The bacterial periplasmic methionine‐binding protein MetQ is involved in the import of methionine by the cognate MetNI methionine ATP binding cassette (ABC) transporter. MetQ, the substrate‐binding protein (SBP) for MetNI,5, 6 is proposed to play a dual role in transport by either binding l‐methionine for delivery to the translocation pathway of MetNI, or by facilitating d‐methionine uptake through the ligand‐free form when complexed to the transporter. Structural studies of SBPs in their ligand‐bound and ligand‐free forms have revealed a hinge‐bending or “Venus‐flytrap” mechanism where two domains of SBPs adopt their open conformation with an accessible binding site in the absence of substrate; substrate binding stabilizes the closed conformation, where the two domains come together and sequester the substrate. In this study, we report the structures of the Neisseria meningitides MetQ in substrate‐free form and in complexes with l‐methionine and with d‐methionine, along with the associated binding constants determined by isothermal titration calorimetry.

MetQ can bind to other methionine derivatives, including d‐methionine, but preparing these forms has been complicated by the high affinity for l‐methionine. Hence, to crystallize the d‐methionine bound N. meningitides MetQ, we developed an alternative approach by unfolding/refolding MetQ during the MetQ purification to remove the endogenous bound l‐methionine. A sample of unfolded/refolded MetQ was then mixed with 10 mM d‐methionine prior to the crystallization. Six molecules are present in the asymmetric unit of the d‐methionine bound MetQ crystal. Not surprisingly, l‐ and d‐methionine bind to the same site, interacting with the same set of conserved residues. This observation is consistent at all six MetQ molecules present in the asymmetric unit. The α‐amino and α‐carboxyl groups of both l‐ and d‐methionine interact with residues R156, N213, and N238 located on one domain of MetQ, while from the other lobe, residues Y81, F98, H100, and Y103 pack around the methionine thioether group. Short contacts to the methionine CB group are observed in both structures, with ∼3.3 å distances observed to the Y98 CO in the l‐methionine structure, and to the Y81 OH groups in the d‐methionine structure. The side chains of l‐ and d‐methionine adopt distinct rotameric conformations for the N‐Cα‐Cβ‐Cγ; Cα‐Cβ‐Cγ‐Sδ; and Cβ‐Cγ‐Sδ‐Cε torsion angles, which are approximately −175°, −175°, and −70° for l‐methionine and +170°, −80°, and −60° for d‐methionine; the latter values correspond to −170°, +80°, and + 60°, respectively, for l‐methionine. Consequently, while there are differences in the details of the binding interactions between l‐ and d‐methionine to NmMetQ, a qualitative evaluation does not identify any obvious feature as dominating the differences in binding affinities for these two ligands.

>KHKEIVFGTTVGDFGDMVKEQIQAELEKKGYTVKLVEFTDYVRPNLALAEGELDINVFQHKPYLDDFKKEHNLDITEVFQVPTAPLGLYPGKLKSLEEVKDGSTVSAPNDPSNFARVLVMLDELGWIKLKDGINPLTASKADIAENLKNIKIVELEAAQLPRSRADVDFAVVNGNYAISSGMKLTEALFQEPSFAYVNWSAVKTADKDSQWLKDVTEAYNSDAFKAYAHKRFEGYKSPAAWNEGAAK[6x]> APSFDCGKPQVEPKKCPGRVVGGCVAHPHSWPWQVSLRTRFGMHFCGGTLISPEWVLTAAHCLEKSPRPSSYKVILGAHQEVNLEPHVQEIEVSRLFLEPTRKDIALLKLSSPAVITDKVI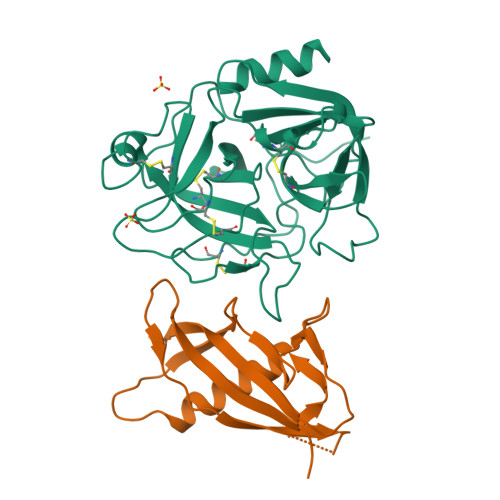PACLPSPNYVVADRTECFITGWGETQGTFGAGLLKEAQLPVIENKVCNRYEFLNGRVQSTELCAGHLAGGTDSCQGDAGGPLVCFEKDKYILQGVTSWGLGCARPNKPGVYVRVSRFVTWIEGVMRNN;> NNSQLVVSVAGTVEGTNQDISLKFFEIDLTSRPASKPFATDSGAMPHKLEKADLLKAIQEQLIANVHSNDDYFEVIDFASDATITDRNGKVYFADKDGSVTLPTQPVQEFLLSGHVRVRPYK> GPLGSMVATVKRTIRIKTQQHILPEVPPVENFPVRQWSIEIVLLDDEGKEIPATIFDKVIYHLHPTFANPNRTFTDPPFRIEEQGWGGFPLDISVFLLEKAGERKIPHDLNFLQESYEVEHVIQIPLNKPLLTEELAKSGST

One of the major and widespread PTMs is acylation of the ε-amino group of lysine residues. Canonical acyllysine readers, bromodomain and double PHD finger (DPF), display comparable binding capabilities toward various short acyl chain modifications, and while the YEATS domain exhibits preference for crotonyllysine, it still associates albeit more weakly with other acyllysine marks. In this study, we elucidate the significance of π stacking components in targeting of acetyllysines by the YEATS domains and report a previously uncharacterized DNA-binding activity of the human AF9-YEATS domain. Collectively, our results have illuminated the mechanistic basis underlying distinct recognition of acyllysine PTMs by the YEATS domains of yeast Taf14 and human AF9, allowing us to develop a Taf14-YEATS module that selects for the crotonyl modification and discriminates against saturated acyl modifications.

In contrast, when complexed with H3K9cr, W81 adopted two conformations, with r1 and r2 providing maximum π stacking with the crotonyl amide and the crotonyl alkene moiety, respectively. Neither the complex with propionylated H3K9pr peptide nor the complex with acetylated H3K9ac peptide had the r2 conformation of W81, indicating that it is a unique feature available to the unsaturated acyl modification but not to saturated acyllysine modifications.> MAAEEGVASAASAGGSWGTAAMGRVLPMLLVPVPAEAMGQLGSRAQLRTQPEALGSLTAAGSLQVLSLTPGSRGGGRCCLEGPFWHFLWEDSRNSSTPTEKPKLLALGENYELLIYEFNLKDGRCDATILYSCSREALQKLIDDQDISISLLSLRILSFHNNTSLLFINKCVILHIIFPERDAAIRVLNCFTLPLPAQAVDMIIDTQLCRGILFVLSSLGWIYIFDVVDGTYVAHVDLALHKEDMCNEQQQEPAKISSFTSLKVSQDLDVAVIVSSSNSAVALNLNLYFRQHPGHLLCERILEDLPIQGPKGVDEDDPVNSAYNMKLAKFSFQIDRSWKAQLSSLNETIKNSKLEVSCCAPWFQDILHLESPESGNHSTSVQSWAFIPQDIMHGQYNVLQKDHAKTSDPGRSWKIMHISEQEEPIELKCVSVTGFTALFTWEVERMGYTITLWDLETQGMQCFSLGTKCIPVDSSGDQQLCFVLTENGLSLILFGLTQEEFLNRLMIHGSASTVDTLCHLNGWGRCSIPIHALEAGIENRQLDTVNFFLKSKENLFNPSSKSSVSDQFDHLSSHLYLRNVEELIPALDLLCSAIRESYSEPQSKHFSEQLLNLTLSFLNNQIKELFIHTEELDEHLQKGVNILTSYINELRTFMIKFPWKLTDAIDEYDVHENVPKVKESNIWKKLSFEEVIASAILNNKIPEAQTFFRIDSHSAQKLEELIGIGLNLVFDNLKKNNIKEASELLKNMGFDVKGQLLKICFYTTNKNIRDFLVEILKEKNYFSEKEKRTIDFVHQVEKLYLGHFQENMQIQSFPRYWIKEQDFFKHKSVLDSFLKYDCKDEFNKQDHRIVLNWALWWDQLTQESILLPRISPEEYKSYSPEALWRYLTARHDWLNIILWIGEFQTQHSYASLQQNKWPLLTVDVINQNTSCNNYMRNEILDKLARNGVFLASELEDFECFLLRLSRIGGVIQDTLPVQNYKTKEGWDFHSQFILYCLEHSLQHLLYVYLDCYKLSPENCPFLEKKELHEAHPWFEFLVQCRQVASNLTDPKLIFQASLANAQILIPTNQASVSSMLLEGHTLLALATTMYSPGGVSQVVQNEENENCLKKVDPQLLKMALTPYPKLKTALFPQCTPPSVLPSDITIYHLIQSLSPFDPSRLFGWQSANTLAIGDAWSHLPHFSSPDLVNKYAIVERLNFAYYLHNGRPSFAFGTFLVQELIKSKTPKQLIQQVGNEAYVIGLSSFHIPSIGAACVCFLELLGLDSLKLRVDMKVANIILSYKCRNEDAQYSFIRESVAEKLSKLADGEKTTTEELLVLLEEGTWNSIQQQEIKRLSSESSSQWALVVQFCRLHNMKLSISYLRECAKANDWLQFIIHSQLHNYHPAEVKSLIQYFSPVIQDHLRLAFENLPSVPTSKMDSDQVCNKCPQELQGSKQEMTDLFEILLQCSEEPDSWHWLLVEAVKQQAPILSVLASCLQGASAISCLCVWIITSVEDNVATEAMGHIQDSTEDHTWNLEDLSVIWRTLLTRQKSKTLIRGFQLFFKDSPLLLVMEMYELCMFFRNYKEAEAKLLEFQKSLETLNTAATKVHPVIPAMWLEDQVCFLLKLMLQQCKTQYELGKLLQLFVEREHLFSDGPDVKKLCILCQILKDTSIAINHTIITSYSIENLQHECRSILERLQTDGQFALARRVAELAELPVDNLVIKEITQEMQTLKHIEQWSLKQARIDFWKKCHENFKKNSISSKAASSFFSTQAHVACEHPTGWSSMEERHLLLTLAGHWLAQEDVVPLDKLEELEKQIWLCRITQHTLGRNQEETEPRFSRQISTSGELSFDSLASEFSFSKLAALNTSKYLELNSLPSKETCENRLDWKEQESLNFLIGRLLDDGCVHEASRVCRYFHFYNPDVALVLHCRALASGEASMEDLHPEIHALLQSAELLEEEAPDIPLRRVHSTSSLDSQKFVTVPSSNEVVTNLEVLTSKCLHGKNYCRQVLCLYDLAKELGCSYTDVAAQDGEAMLRKILASQQPDRCKRAQAFISTQGLKPDTVAELV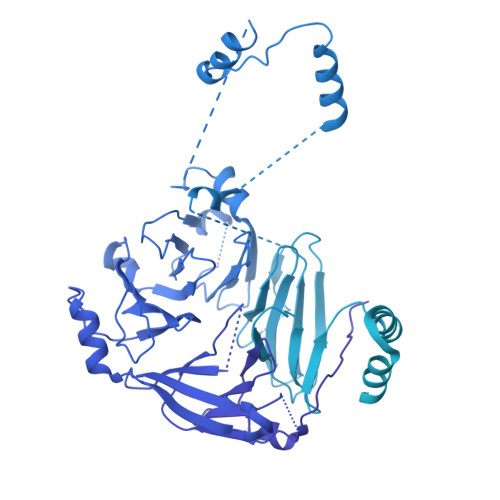AEEVTRELLTSSQGTGHKQMFNPTEESQTFLQLTTLCQDRTLVGMKLLDKISSVPHGELSCTTELLILAHHCFTLTCHMEGIIRVLQAAHMLTDNHLAPSEEYGLVVRLLTGIGRYNEMTYIFDLLHKKHYFEVLMRKKLDPSGTLKTALLDYIKRCRPGDSEKHNMIALCFSMCREIGENHEAAARIQLKLIESQPWEDSLKDGHQLKQLLLKALTLMLDAAESYAKDSCVRQAQHCQRLTKLITLQIHFLNTGQNTMLINLGRHKLMDCILALPRFYQASIVAEAYDFVPDWAEILYQQVILKGDFNYLEEFKQQRLLKSSIFEEISKKYKQHQPTDMVMENLKKLLTYCEDVYLYYKLAYEHKFYEIVNVLLKDPQTGCCLKDMLAG>MKRAVITGLGIVSSIGNNQQEVLASLREGRSGITFSQELKDSGMRSHVWGNVKLDTTGLIDRKVVRFMSDASIYAFLSMEQAIADAGLSPEAYQNNPRVGLIAGSGGGSPRFQVFGADAMRGPRGLKAVGPYVVTKAMASGVSACLATPFKIHGVNYSISSACATSAHCIGNAVEQIQLGKQDIVFAGGGEELCWEMACEFDAMGALSTKYNDTPEKASRTYDAHRDGFVIAGGGGMVVVEELEHALARGAHIYAEIVGYGATSDGADMVAPSGEGAVRCMKMAMHGVDTPIDYLNSHGTSTPVGDVKELAAIREVFGDKSPAISATKAMTGHSLGAAGVQEAIYSLLMLEHGFIAPSINIE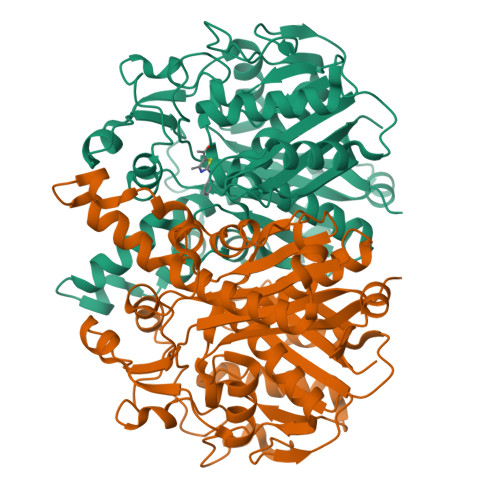ELDEQAAGLNIVTETTDRELTTVMSNSFGFGGTNATLVMRKLKD[4x]> MATAEVLNIGKKLYEGKTKEVYELLDSPGKVLLQSKDQITAGNAARKNHLEGKAAISNKITSCIFQLLQEAGIKTAFTRKCGETAFIAPQCEMIPIEWVCRRIATGSFLKRNPGVKEGYKFYPPKVELFFKDDANNDPQWSEEQLIAAKFCFAGLLIGQTEVDIMSHATQAIFEILEKSWLPQNCTLVDMKIEFGVDVTTKEIVLADVIDNDSWRLWPSGDRSQQKDKQSYRDLKEVTPEGLQMVKKNFEWVAERVELLLKSESQCRVVVLMGSTSDLGHCEKIKKACGNFGIPCELRVTSAHKGPDETLRIKAEYEGDGIPTVFVAVAGRSNGLGPVMSGNTAYPVISCPPLT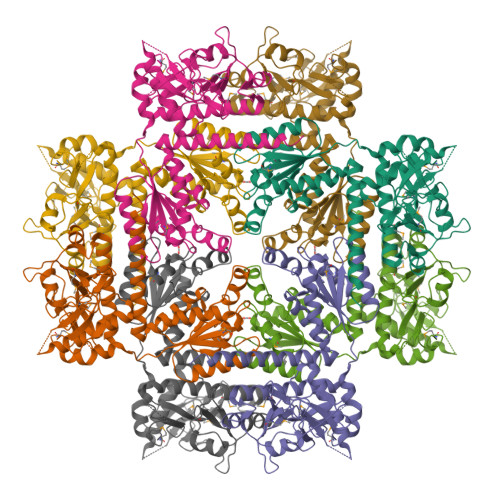PDWGVQDVWSSLRLPSGLGCSTVLSPEGSAQFAAQIFGLSNHLVWSKLRASILNTWISLKQADKKIRECNL> MPKALRFLGWPVLVGVLLALLIIQHNPELVGLPRQEVHVEQAPLLSRLQEGPPSYANAVSRAAPAVANLYTTKMVSKPSHPLFDDPMFRRFFGDNLPQQKRMESSLGSAVIMSAEGYLLTNNHVTAGADQIIVALRDGRETIAQLVGSDPETDLAVLKIDLKNLPAMTLGRSDGIRTGDVCLAIGNPFGVGQTVTMGIISATGRNQLGLNTYEDFIQTDAAINPGNSGGALVDAAGNLIGINTAIFSKSGGSQGIGFAIPTKLALEVMQSIIEHGQVIRGWLGVEVKALTPELAESLGLGETAGIVVAGVYRDGPAARGGLLPGDVILTIDKQEASDGRRSMNQVARTRPGQKISIVVLRNGQKVNLTAEVGLRPPPAPAPQQKQDGGE;> WVF

AlgW, a membrane-bound periplasmic serine protease belonging to the HtrA protein family, is a key regulator of the regulated intramembrane proteolysis (RIP) pathway and is responsible for transmitting the envelope stress signals in Pseudomonas aeruginosa. The AlgW PDZ domain senses and binds the C-terminal of mis-localized outer membrane proteins (OMPs) or periplasmic protein MucE, leading to catalytic activation of the protease domain. HtrA protease is characterized by its trypsin-like catalytic domain and regulatory PDZ domain; the catalytic triad was surrounded by several loops (L1, L2, L3, LD, LA) but, usually, in an inactive mode, and could be activated by sensing a specific molecular stimulus. The catalytic triad (H123, D153, and S227) sites are located between two β-barrels and are surrounded by activation loops L1 to L3, LD, and LA (named according to DegS nomenclature).

Protein samples were mixed with two types of peptide activator (tripeptide WVF, decapeptide SVRDELRWVF) prior to crystallization trials, yielding four complex structures, AlgW-tripeptide, AlgWS227A-tripeptide, AlgW-decapeptide, and AlgWS227A-decapeptide, with resolutions from 1.8 to 2.6 Å. AlgW-tripeptide and AlgWS227A-tripeptide crystals belong to the P6322 space group. They have only one complex in an asymmetric unit, and their overall structures are similar (the root mean square deviation [RMSD] value was 1.07 Å). The AlgW trimer could be generated by symmetry operation, and similar to most HtrA protease, this funnel-like trimeric organization is mainly mediated by the N-terminal protease domains. Because of the high flexibility, our AlgW-tripeptide and AlgWS227A-tripeptide structures, as well as many HtrA protease structures, lack the LA loops. AlgW and DegS share similar hydrophobic environments to accommodate the large side chains of aromatic residues 0 and –2 (for instance, WVF for AlgW and YQF for DegS) in peptide activators. Consistently, AlgW-peptide bound structures also demonstrated different interdomain orientations, in which the joint angles of the PDZ relative to the protease domain are AlgW-WVF (25.62°) < AlgWS227A-WVF (25.74°) < AlgW-decapeptide (25.47 to 26.48°; average, 26.13°) < AlgWS227A-decapeptide (26.65°). Thus, by recognizing additional C-terminal residues of the targeting protein, the PDZ domain of AlgW adopts a more open form and maintains a more stable state, generating stronger substrate cleavage activity. This is in accordance with our enzymatic assay in which the tripeptide-bound AlgW is partially activated, while the decapeptide-bound structures reflect the further activation of AlgW.> MEVTVPDALKDRIALKKTARQLNIVYFLGSDTEPVPDYERRLSELLLYLQQFYGKEMQRHGYGARSFGLDIKSPGRVNIIEYKAKNPAAHYPYENGGGWKAAQELDEFFKAHPDRKKSQHTLIIMPTWNDEKNGPDNPGGVPFYGMGRNCFALDYPAFDIKHLGQKTREGRLLTKWYGGMAAALGHGLNLPHNHQTASDGKKYGTALMGSGNYTFGTSPTFLTPASCALLDACEVFSVTPSQQFYEGKPE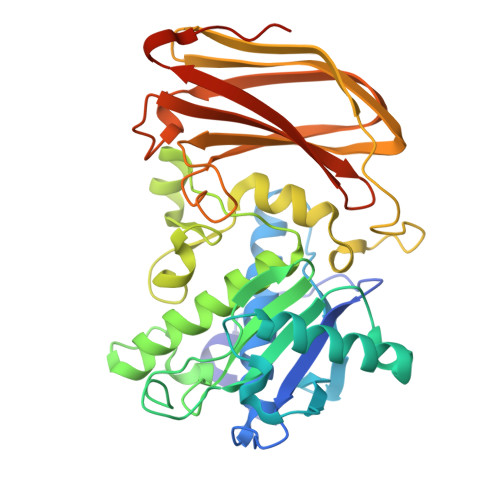VEVGDVAISFKGDQILVSGNYKSPQTVKALNVYIQDPPYAVNQDYDAVSFSRRLGKKSGKFSMKIDKKELEGLNNNEFRISLMFILANGLHMQKHFTFHWDALQDYRDGSKSGSGHHHHHH>GESLFKGPRDYNPISSTICHLTNESDGHTTSLYGIGFGPFIITNKHLFRRNNGTLLVQSLHGVFKVKNTTTLQQHLIDGRDMIIIRMPKDFPPFPQKLKFREPQREERICLVTTNFQTKSMSSMVSDTSCTFPSSDGIFWKHWIQTKDGQAG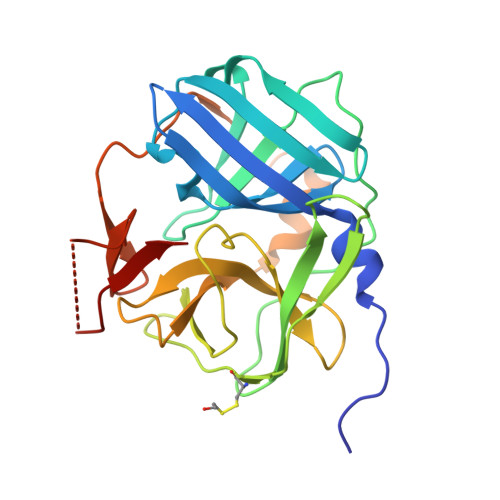SPLVSTRDGFIVGIHSASNFTNTNNYFTSVPKNFMELLTNQEAQQWVSGWRLNADSVLWGGHKVFMSKPEEPFQPVKEATQLMNELVYSQ[2x]> APAKPDHAATQQALEAAVADGVPGAVAQARDGRDRWTGTAGERGGDDRYRVGSITKTFTATVLLQLQAEGRI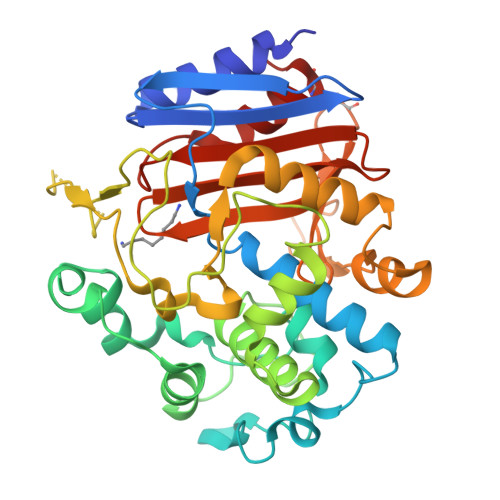DLDDPVEKWLPGVVRGNGHDGRKITVRQLLNHTSGIYSYTEDPAFQAKVFGPGFLEHRYDTWTPKQLVAVAMAHEPDFTPGASWNYSNTNFVLAGMVIEKVTGRPYGKAVENRIIKPLKLRATTVPGTRSAMPEPSSPAYSKLSRDVNAPVHDVSTLNPSIAGAAGEMISDSRDLQTFYRALLQGRLLPKSALNEMTTTVQISPEYPNVGYGLGLMKDKLSCGVEVWGHGGGIHGSSSLAQVTRDGGHSLAGNFNADWAGDSQKVIEAEFCGTAPKK>SNGGFCEVCKKLVLYLEHNLEKNSTKEEILAALEKGCSFLPDPYQKQCDDFVAEYEPLLLEILVEVMDPGFVCSKIGVCPSAY[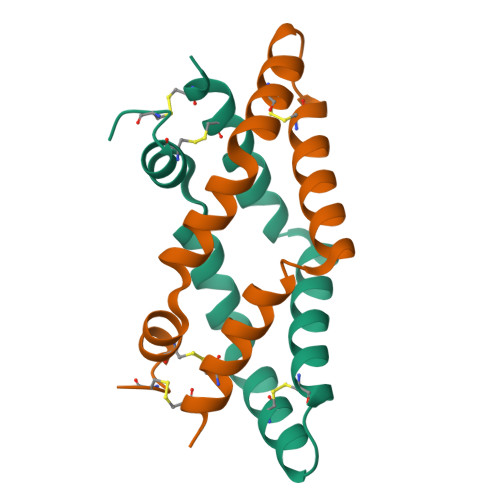2x]>[2x]MRGSHHHHHHGLVPRGSMIRTMLQGKLHRVKVTHADLHYEAGSCAIDQDFLDAAGILENEAIDIWNVTNGKRFSTYAIAAERGSRIISVNGAAAHCASVGDIVII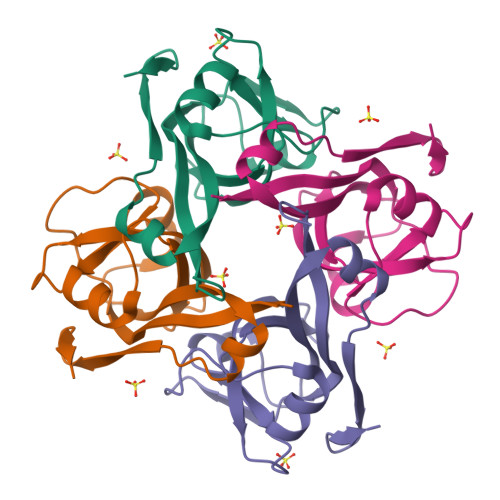ASFVTMPDEEARTWRPNVAYFEGDNEMKRTAKAIPVQVA>[6x]MNNEIGRKITSLTLMTIMVAGGLTFAIPG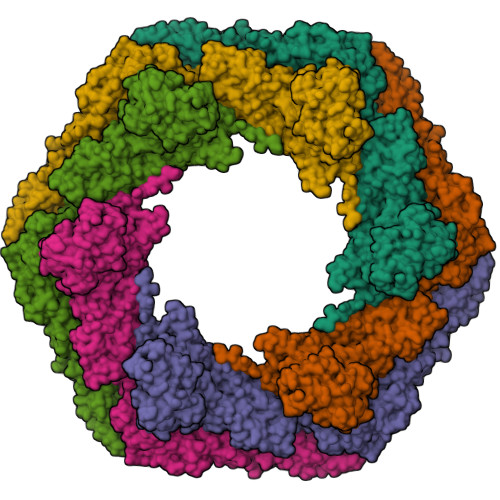VMPEAMAANANLFVSAENSQFDNYMSGPQVIEVVVIDSDINDTDEAKGEPDVTVNGKVLRMVQAVDGNWYGYFADRDQAQIADSTATTADSGLDFGVFCASSSGTAALGFSTTETDGIAIPITIANATATGNGTQTGSSSGGAITTTCAANTLDASTANGTINVVREAKDPVAASGSVSVGQIGLKNGTANSGPNWPFIQLYELNPTGNVVVQYNKGGGVQSTTLTFDTVDQFAELSLDRTVFPRVSQVHATITDLWLNIDPTDEDSWTFATNTKNTTSSFNVDTFYQVFDENGASGGSALTLRTTLSSLMCEDNCVLTLDVDAQSSGTPVVTIQDNGDSILTQLNASSNTNANNASAFGISTETAKLGTGSIPVTITEQGPNSGVFGTYDESDKSVLKITDNAKRGTSASLDYNETPQTILVGFSFASIDIQPVTDEWTSGQEIPVVIVDADQNKNSRADEDLDLNNPDVTLIPALRTGDPFTIDEGGTPSLIFTNGTNGDDSIFDTGAINNTSAGQVGNFTLNINVTRFSSATNITSTESIDTFSKRLISAQTANSSANFDVDFAIIDLGSATLETLKETVVDEDNTAVGFNFFNYDVRSLGADTVSIALLNTTGNILPWVNNDTRNVDKNNAILLVSNSTNSQAYVDLTNAVSDAVYGSTNTDSNVNIGFAMYFTGVGDLAAKEVIVMDFFSFGFTDDGVQSSERFANQIIRIEAEETGDNTSTFEGSLEYVMVNQINIQDAGTFSGITPIADDPSFIVIEDLTDEDAPRVNYNDLGADGVTTPVSDQEEAPSHSGVVSLNADSYKIADTVVITVEDLDLNVDSDLIDIFTVVSDNSKATDDAVGSATTQSLSFGELGRLLDVTFDDVIWSTPDGANNTATGNDSDTCSTELSNAGITDTGLGATGFTLVETGAATGVFVGDFQIPSFWCRVSDTTTTPYTYAGDEETTTGLDIEVNYVDFRDASGEIVEVGDSAGVRANTGSVSLDRTVYPVPFGTIADSSKAANAAPNGRSVFPIHATGITSTIDSTEELPTGDLTIHVRINDPDFDENPAGEDAMDQDNALKISVIRGSDSVVLGYAGASERTGKIDVGGNNGTISNIRSFGEMDEIAPDAGIFELDVNIKFTDGPASAQCNSHDTLYTALDGTTGKADTNRFDDGAASGQEYCILQGDILQVEYTDPADASGDANTVTDSATFDLRNGVLQSDKSVYIIGSDMILTLIEPDFDLDNDSAETYDLDLIEWDSDAATTTMGNKGVTGAAAAFDPEPTDFRETGDSTGIFQIVIEIPESLSNDKLERGEEIILEYTDWGPSGSDYVGDEDEDVNLTIYTSNFGATVELDQKVYSWTDKVYITIVAPDHNFDSDLVDEIGETDSDPIKVSTRGFDLDNYKLVETGTDTGIFTGEVILTGFTAHDADGDGNTGDATGTTSGSGPTDGLLATDDDDGLTVSFEFSEDETIVGSALIRWNIGEVQWLEASYPASGTGVVRVIDPDMNLDPEAVDNFEVDVWSDSDAGGIDLTVTETNEATGIFEGTVFFTTLDESSGHRLRVSEGDTVTAEYEDNTLPDPYTTADELDITATSLIGTVVPPLERAPAANLRTVDAFGNSLDSVSVDQQVQISADLANGQDREQSFAYLVQIQDANGVTVSLAWITGSLSSGQSFSPALSWIPTEAGTYTATAFVWESVDNPTALSPPVSTTVNVS> SEGNGPAAVHYQPASPPRDACVYSSCYCEENVWKLCEYIKNHDQYPLEECYAVFISNERKMIPIWKQQARPGDGPVIWDYHVVLLHVSSGGQSFIYDLDTVLPFPCLFDTYVEDAIKSDDDIHPQFRRKFRVICADSYLKNFASDRSHMKDS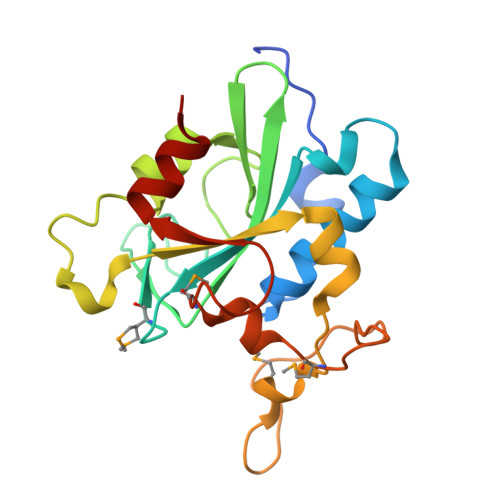SGNWREPPPPYPCIETGDSKMNLNDFISMDPKVGWGAVYTLSEFTHRFGSKNC We had previously identified the transcription factor FasR, as a key activator of fas and acpS gene expression. fas and acpS, respectively, coding for FAS I synthase and 4-phosphopantetheinyl transferase (essential to produce functional ACP), form a single operon in Mtb. FasR:DNA binding is regulated by long-chain acyl-CoAs, which are themselves products of FAS I, namely acyl-CoAs ≥ C16 disrupt the interaction of Mtb FasR with its cognate DNA6. FasR is a TFR member that senses long and very long acyl-CoA moieties, subsequently turning off FAS I-mediated fatty acid biosynthesis. We have now determined the 3D structures of FasR from Mtb, in three different states obtained with the protein (i) crystallised alone, (ii) co-crystallised in complex with the fatty acid C20-acyl-CoA and (iii) in complex with a double-stranded DNA oligonucleotide bearing the specific FasR-binding sequence.

FasRΔ33 crystals were also grown in the absence of acyl-CoA with the aim of solving the ligand-free structure. Unexpectedly, additional electron density not corresponding to protein, was visible within the ligand-binding tunnel. The density is also consistent with myristic acid (C14), which we hypothesize could likely bind during protein expression in E. coli. Even if the chemical nature of the bound species is not certain, this piece of evidence results in two consequences: FasRΔ33-C14 is not a true apo form of the protein, but it did disclose by serendipity the structure of FasR with a shorter alkyl chain bound in the effector pocket, as compared with FasRΔ33-C20-CoA. In contrast to the strictly symmetric organization of the FasRΔ33-C20-CoA dimer, FasRΔ33-C14 displays one full dimer per asymmetric unit, each protomer deviates from strict symmetry with respect to the other. The HTH domains of FasRΔ33-C14 depart from this relationship, after superimposing one protomer onto the other, the EBDs fit together well, while the HTHs are rotated by ~15°. Departure from intradimer symmetry is thus largely due to substantial flexibility in the region that joins the regulatory and the DNA-binding domains, not the hinge loop covalently linking both domains, but rather the whole region involving the HTH as a rigid domain plus the lower part of the regulatory domain’s helices that interact with the HTH (mainly the N-terminal half of α4). Using the position of conserved Tyr77 Cα as a reference (at the centre of helix α3, key to mediate DNA-binding), the two HTH domains in FasRΔ33-C14 are ~48 Å apart, vs ~57 Å in FasRΔ33-C20-CoA. In contrast, when the tunnel is occupied with a too short acyl chain, greater HTH mobility is enabled, allowing helices α3 to reach a proper separation distance to binding DNA (ideal B-DNA has 34 Å separation between major grooves on the same side of the double helix).

>[2x]FQGMLPRDERRGQLLVVASDVFVDRGYHAAGMDEIADRAGVSKPVLYQHFSSKLELYLAVLHRHVENLVSGVHQALSTTTDNRQRLHVAVQAFFDFIEHDSQGYRLIFENDFVTEPEVAAQVRVATESCIDAVFALISADSGLDPHRARMIAVGLVGMSVDCARYWLDADKPISKSDAVEGTVQFAWGGLSHVPL>MKVGIVGSGMVGSATAYALALLGVAREVVLVDLDRKLAQAHAEDILHATPFAHPVWVWAGSYGDLEGARAVVLAAGVAQRPGETRLQLLDRNAQVFAQVVPRVLEAAPEAVLLVATNPVDVMTQVAYALSGLPPGRVVGSGTILDTARFRALLAEYLRVAPQSVHAYVLGEHGDSEVLVWSSAQVGGVPLLEFAEARGRALSPEDRARIDEGVRRAAYRIIEGKGATYYGIGAGLARLVRAILTDEKGVYTVSAFTPEVAGVLEVSLSLPRILGAGGVAGTVYPSLSPEERAALRRSA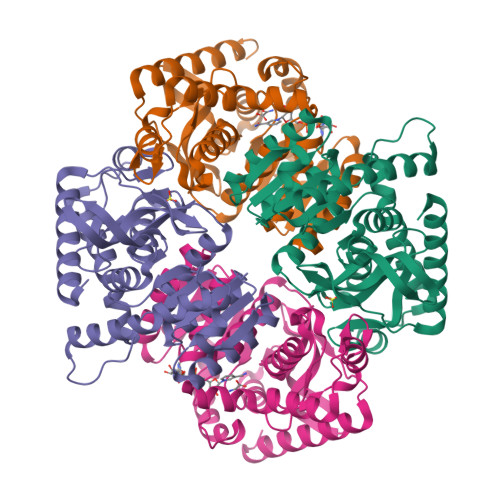EILKEAAFALGF[4x]>[6x]GSMKKEFTELYDFIFDPIFLVRYGYYDRSIKNKKMNTAKVELDNEFGKSDSFYFKVFNMESFADYLRSHDLKTHFNGKKPLSTDPVYFNIPKNIEARRQYKMPNLYSYMALNYYICD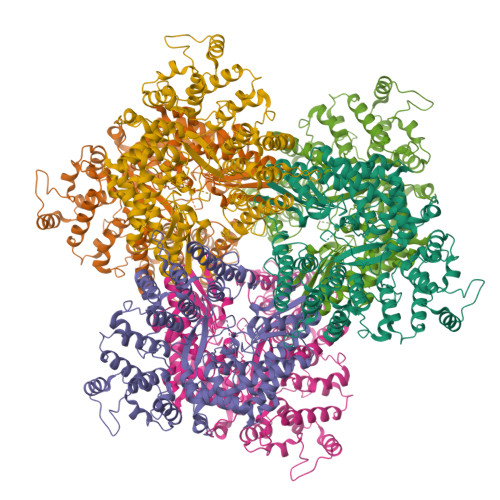NKKEFIEVFIDNKFSTSKFFNQLNFDYPKTQEITQTLLYGGIKKLHLDLSNFYHTLYTHSIPWMIDGKSASKQNRKKGFSNTLDTLITACQYDETHGIPTGNLLSRIITELYMCHFDKQMEYKKFVYSRYVDDFIFPFTFENEKQEFLNEFNLICRENNLIINDNKTKVDNFPFVDKSSKSDIFSFFENITSTNSNDKWIKEISNFIDYCVNEEHLGNKGAIKCIFPVITNTLKQKKVDTKNIDNIFSKRNMVTNFNVFEKILDLSLKDSRLTNKFLTFFENINEFGFSSLSASNIVKKYFSNNSKGLKEKIDHYRKNNFNQELYQILLYMVVFEIDDLLNQEELLNLIDLNIDDYSLILGTILYLKNSSYKLEKLLKKIDQLFINTHANYDVKTSRMAEKLWLFRYFFYFLNCKNIFSQKEINSYCQSQNYNSGQNGYQTELNWNYIKGQGKDLRANNFFNELIVKEVWLISCGENEDFKYLN> MMQNLKKFMSKTIQVQPVSFNQIPKAFYNFPEYRTGGVQANPGITAKRIIKCIGERLRKYDPARWENVPITFKTHFRDENGYSDVATSIQIHDALEREFGIDI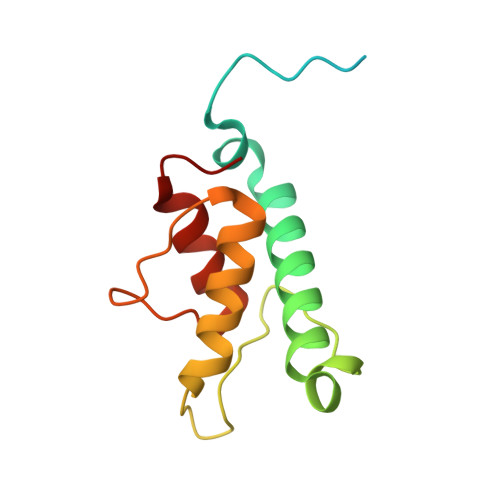KDRLALVTDVETAFYIVMSHHDPL N-(2-isopropoxy-4-(4-methylpiperazine-1-carbonyl)phenyl)-2-(3-(3-phenylureido)phenyl)thiazole-4-carboxamide 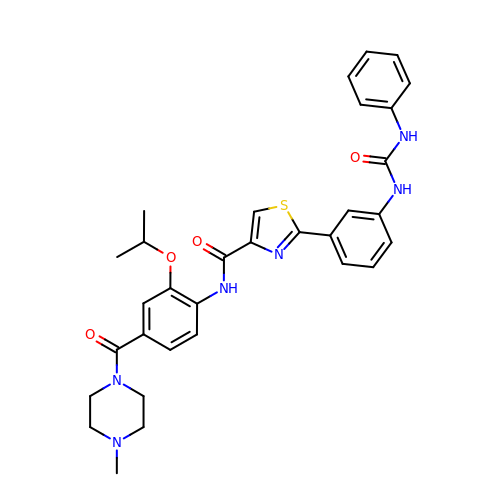| C32 H34 N6 O4 S | YHONMSVJCMGHMF-UHFFFAOYSA-N> HLELTEEQKAKVKVHFDECVKQEKVSEEEATKLRNKDYANPTPAMKCFGTCFFEKI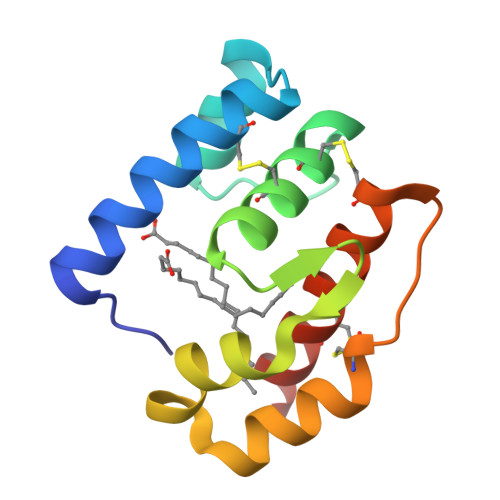GTLKDGVVQEAVVLEKLSPHFGEEKVKAALDKCKNIKGADRCDTGFKIFECFEKAKDELGH> AMALEQALQAARRGDLDVLRSLHAAGLLGPSLRDSLDALPVHHAARSGKLHCLRYLVEEVALPAVSRARNGATPAHDAAATGYLSCLQWLLTQGGCRVQEKDNSGATVLHLAARFGHPDVVKWLLYQGGANSAITTDTGALPIHYAAAKGDLPSLKLLVGHYPEGVNAQTNNGATPLYLACQEGHLEVTKYLVQECSADPHLRAQDGMTPLHAAAQMGHNPVLVWLVSFADVSFSEQDHDGATAMHFAASRGHTKVLSWLLLHGAEISQDLWGGTPLHDAAENGELECCQILAVNGAGLDVRD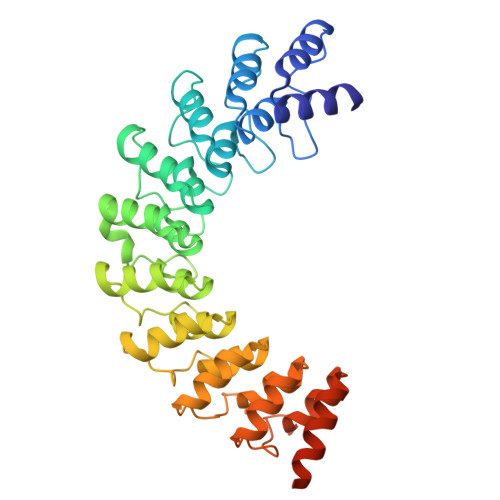HDGYTAADLAEFNGHTHCSRYLRTVQTLSLEHRVLSRDQSMDLEAKQLDS4-[3-AMINO-6-(3-ETHYLTHIOPHEN-2-YL)PYRAZIN-2-YL]CYCLOHEXANE-1-CARBOXYLIC ACID | C17 H21 N3 O2 S | 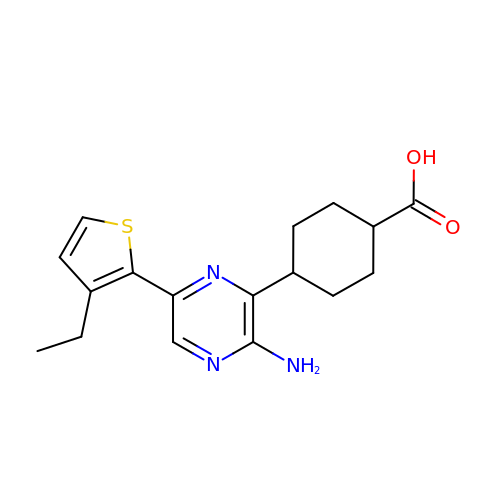QTTNDIPJKXHHFL-HAQNSBGRSA-N> AVTHH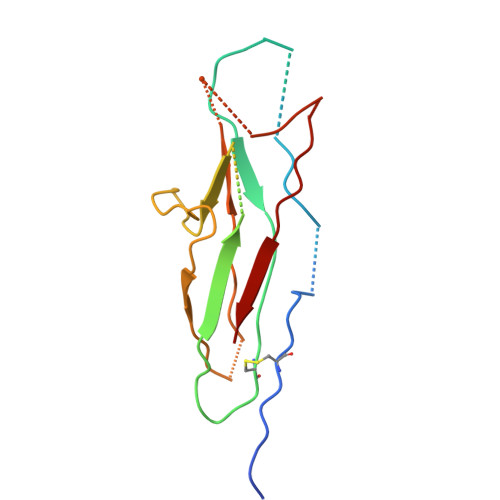HHHHSTGCTVGGSQTEGNMNKFGTLNFGKTSGTWNNVLTAEVASAATGGNISVTCDGTDPVDFTVAIDGGERTDRTLKNTASADVVAYNVYRDAARTNLYVVNQPQQFTTVSGQATAVPIFGAIAPNTGTPKAQGDYKDTLLVTVNF> QPQFNEDTLQQRLQALIESAGENWTYAIFWQISHDFDSSTGDNTVILGWGDGYYKGEEDKEKKKNNT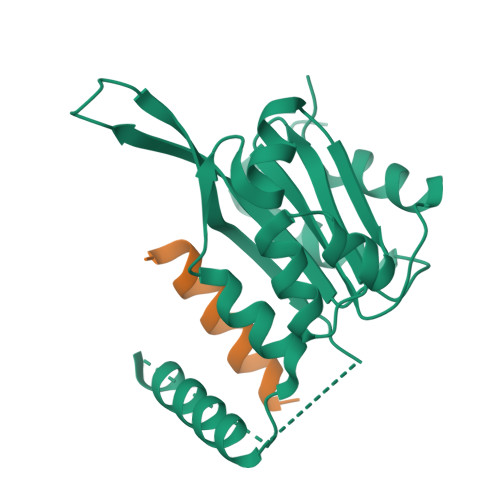NTAEQEHRKRVIRELNSLISGGIGVSDESNDEEVTDTEWFFLVSMTQSFVNGVGLPGESFLNSRVIWLSGSGALTGSGCERAGQGQIYGLKTMVCIATQNGVVELGSSEVISQSSDLMHKVNNLFNFNNGGG;> DLPIARRKSLQRFLEKRKERLVSTSPY> MQPGATTCTEDRIQHALERCLHGLSLSRRSTSWSAGLCLNCWSLQELVSRDPGHFLILLEQILQKTREVQEKGTYDLLAPLALLFYSTVLCTPHFPPDSDLLLKAARTYHRFLTWPVPYCSICQELLTFIDAELKAPGISYQRLVRAEQGLSTRSHRSSTVTVLLLNPVEVQAEFLDVADKLSTPGPSPHSAYITLLLHAFQATFGAHCDLSGLHRRLQSKTLAELEAIFTETAEAQELASGIGDAAEARQWLRTKLQAVGEKAGFPGVLDTAKPGKLRTIPIPVARCYTYSWNQDSFDILQEILLKEQELLQPEILDDEEDEDEEDEEEDLDADGHCAERDSVLSTGSAASHASTLSLASSQASGPTLSRQLLTSFVSGLSDGVDSGYMEDIEESAYERPRRPGGHERRGHRRPGQKFNRIYKLF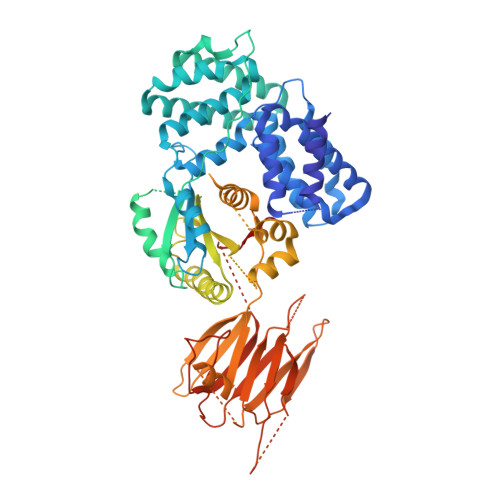KSTSQMVLRRDSRSLEGSPDSGPPLRRAGSLCSPLDSPTLPPSRAQRSRSLPQPKLSPQLPGWLLAPASRHQRRRPFLSGDEDPKASTLRVVVFGSDRISGKVARAYSNLRRLENNRPLLTRFFKLQFFYVPVKRSRGTGTPTSPAPRSQTPPLPTDAPRHPGPAELGAAPWEESTNDISHYLGMLDPWYERNVLGLMHLPPEVLCQSLKAEPRPLEGSPAQLPILADMLLYYCRFAARPVLLQVYQTELTFITGEKTTEIFIHSLELGHSAATRAIKASGPGSKRLGIDGDREAVPLTLQIIYSKGAISGRSRWSNMEKLCTSVNLSKACRQQEELDSSTEALTLNLTEVVKRQTPKSKKGFNQISTSQIKVDKVQIIGSNSCPFAVCLDQDERKILQSVIRCEVSPCYKPEKSSLCPPPQRPSYPPAPATPDLCSLLCLPIMTFSGALPGGGGSDYKDDDDK> SGPINDTDANP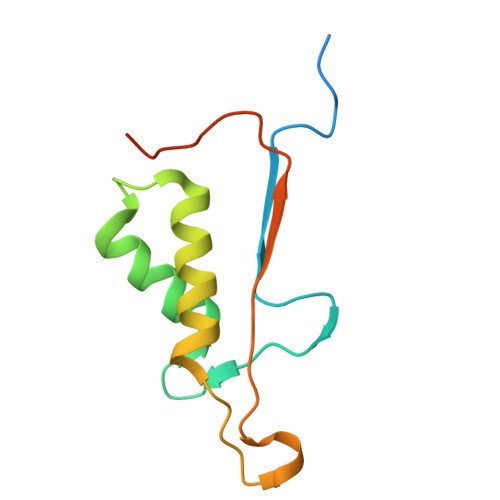RYKIPVEADFLFAYSTVPGYYSWRSPGRGSWFVQALCSILEEHGKDLEIMQILTRVNDRVARHFESQSDDPHFHEKKQIPCVVSMLTKELYFSQLEHHHHHH>[2x]MATANVAGAGGSGSEPTRIAILGKEDIIVDHGIWLNFVAHDLLQTLPSSTYVLITDTNLYTTYVPPFQAVFEAAAPRDVRLLTYAIPPGEYSKSRETKAEIEDWMLSHACTRDTVIIALGGGVIGDMIGYVAATFMRGVRFVQVPTTLLAMVDSSIGGKTAIDTPMGKNLIGAFWQPRRIYIDLAFLETLPVREFINGMAEVIKTAAIWNETEFTALEENAAAILEAVRSKASSPAARLAPIRHILKRIVLGSARVKAEVVSADEREGGLRNLLNFGHSIGHAYEAILAPQVLHGECVAIGMVKEAELARYLGVLRPSAVARLTKLIASYDLPTSVHDKRIAKLSAGKECPVDVLLQKMAVDKKNEGRKKKIVLLSAIGKTYEKKATVVDDRAIRLVLSPSVRVTPGVPKGLSVTVTPPGSKSISNRALVLAALGEGTTRIHGLLHSDDVQYMLAAIEQLHGADFSWEDAGEILVVTGKGGKLQASKEPLYLGNAGTASRFLTSVVALCAPSAVSSTVLTGNARMKVRPIGALVDALRANGVGVKYLEKEKSLPVEVDAAGGFAGGVIELAATVSSQYVSSILMAAPYAHQPVTLRLVGGKPISQPYIDMTIA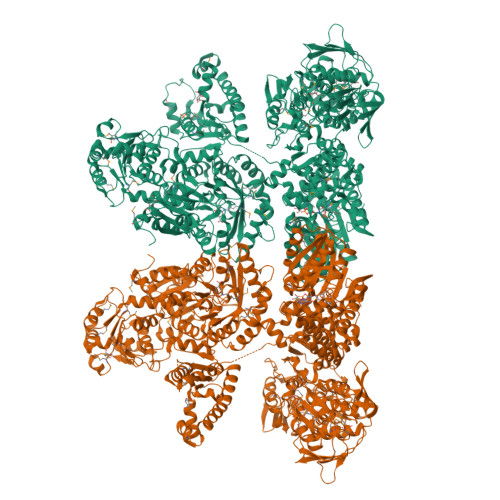MMASFGIKVERSAEDPNTYLIPKGVYKNPPEYVVESDASSATYPLAVAAITGTTCTIPNIGSESLQGDARFAVEVLRPMGCAVEQTATSTTVTGPPIGTLKAIPHVDMEPMTDAFLTAAVLAAVADGTTQITGIANQRVKECNRIAAMKDQLAKFGVQCNELEDGIEVIGKPYQELRNPVEGIYCYDDHRVAMSHSVLSTISPHPVLILERECTAKTWPGWWDILSQFFKVQLDGEEDPTKRTTQSTQQVRKGTDRSIFIVGMRGAGKSTAGRWMSELLKRPLVDLDAELERREGMTIPEIIRGERGWEGFRQAELELLQDVIKNQSKGYIFSCGGGIVETEAARKLLIDYHKNGGPVLLVHRDTDQVVEYLMRDKTRPAYSENIREVYERRKPWFYECSNLQYHSPHEDGSEALLQPPADFARFVKLIAGQSTHLEDVRAKKHSFFVSLTVPNVADALDIIPRVVVGSDAVELRVDLLESYEPEFVARQVALLRAAAQVPIVYTVRTQSQGGKFPDEDYDLALRLYQTGLRSGVEYLDLEMTMPDHILQAVTDAKGFTSIIASHHDPQCKLSWKSGSWIPFYNKALQYGDVIKLVGVAREMADNFALTNFKAKMLAAHDNKPMIALNMGTAGKLSRVLNGFLTPVSHPALPSKAAPGQLSATEIRQALSLIGEIEPKSFYLFGKPISASRSPALHNTLFYKTGLPHHYSRFETDEASKALESLIRSPDFGGASVTIPLKLDIMPLLDSATDAARTIGAVNTIIPQTRDGSTTTLVGDNTDWRGMVHALLHSSGSGSVVQRTAAPRGAAMVVGSGGTARAAIYALHDLGFAPIWIVARSEERVAELVRGFDGYDLRRMTSPHQGKDNMPSVVISTIPATQPIDPSMREVIVEVLKHGHPSAEGKVLLEMAYQPPRTPLMTLAEDQGWRTVGGLEVLAAQGWYQFQLWTGITPLYEEARAAVMGEDSVELEHHHHHH>[2x]TLSILVAHDLQRVIGFENQLPWHLPNDLKHVKKLSTGHTLVMGRKTFESIGKPLPNRRNVVLTSDTSFNVEGVDVIHSIEDIYQLPGHVFIFGGQTLFEEMIDKVDDMYITVIE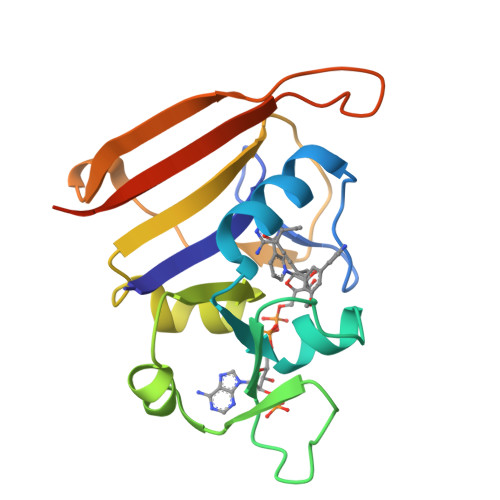GKFRGDTFFPPYTFEDWEVASSVEGKLDEKNTIPHTFLHLIRKLEHHHHHHHH>MRVGIPTETKNNEFRVAITPAGVAELTRRGHEVLIQAGAGEGSAITDADFKAAGAQLVGTADQVWADADLLLKVKEPIAAEYGRLRHGQILFTFLHLAASRACTDALLDSGTTSIAYETVQTADGALPLLAPMSEVAGRLAAQVGAYHLMRTQGGRGVLMGGVPGVEPADVVVIGAGTAGYNAARIANGMGATVTVLDINIDKLRQLDAEFCGRIHTRYSSAYELEGAVKRADLVIGAVLVPGAKAPKLVSNSLVAHMKPGAVLVDIAIDQGGCFEGSRPTTYDHPTFAVHDTLFYCVANMPASVPKTSTYALTNATMPYVL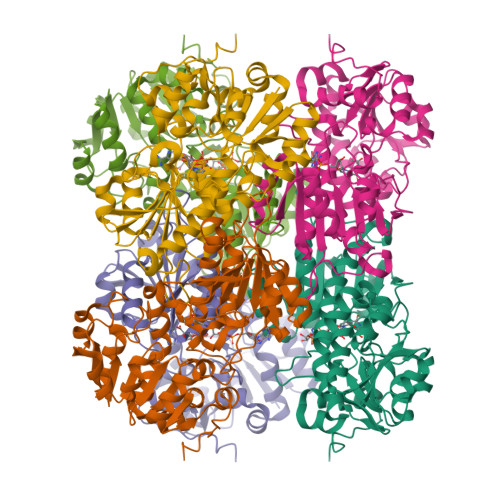ELADHGWRAACRSNPALAKGLSTHEGALLSERVATDLGVPFTEPASVLA[3x]> YQQDQVVKEDNIEAVGKKLHEYNTQFQEKSREYDRL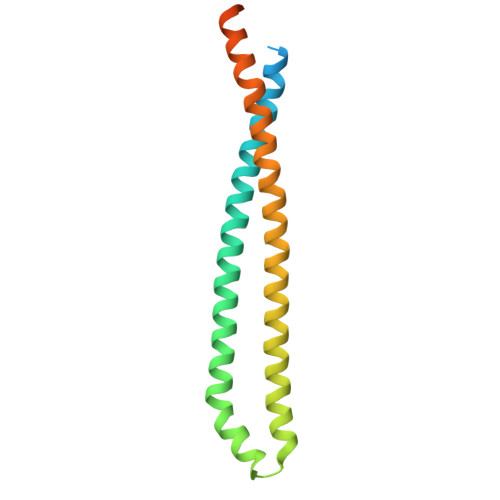YEDYTRTSQEIQMKRTAIEAFNETIKIFEEQCQTQERYSKEYIEKFKREGNETEIQRIMHNYEKLKSRISEIVDSRRRLEEDLKKQAAEYREIDKRMNSIKPDLIQLRKTRDQYLMWLTQKGVRQKKLNEWLG> MRRHYRDLIRNTPMPDTPQDIADLRALLDEDEAEMSVVFSDPSQPDNPAIYVSDAFLVQTGYTLE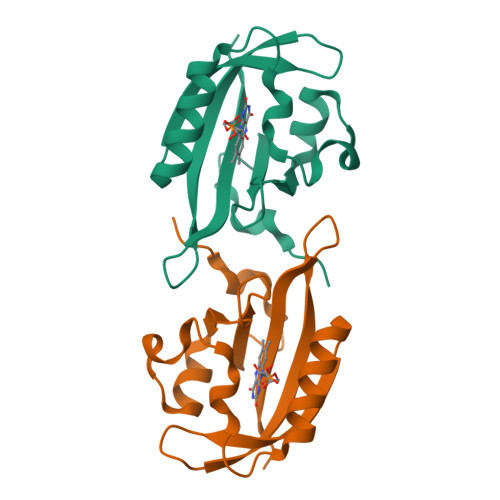EVLGRNCRFLQGPDTNPHAVEAIRQGLKAETRFTIDILNYRKDGSAFVNRLRIRPIYDPEGNLMFFAGAQNPVLEHHHHHH>MLAVPNMRFGIFLLWWGWVLATESRMHWPGREVHEMSKKGRPQRQRREVHEDAHKQVSPILRRSPDITKSPLTKSEQLLRIDDHDFSMRPGFGGPAIPVGVDVQVESLDSISEVDMDFTMTLYLRHYWKDERLSFPSTNNLSMTFDGRLVKKIWVPDMFFVHSKRSFIHDTTTDNVMLRVQPDGKVLYSLRVTVTAMCNMDFSRFPLDTQTCSLEIESYAYTEDDLMLYWKKGNDSLKTDERISLSQFLIQEFHTTTKLAFYSSTGWYNRLYINFTLRRHIFFFLLQTYFPATLMVMLSWVSFWIDRRAVPARVPLGITTVLTMSTIITGVNASMPRVSYIKAVDIYLWVSFVFVFLSVLEYAAVNYLTTVQERKEQKLREKLPCTSGLPPPRTAMLDGNYSDGEVNDLDNYMPENGEKPDRMMVQLTLASERSSPQRKSQRSSYVSMRIDTHAIDKYSRIIFPAAYILFNLIYWSIFS[5x]

The family of ρ-type GABAA receptors includes potential therapeutic targets in several neurological conditions, and features distinctive pharmacology compared to other subtypes. Channels in this family share a common architecture, with each of the five subunits contributing to an extracellular domain (ECD) with 10 strands (β1–β10) and a transmembrane domain (TMD) with 4 helices (M1–M4). The orthosteric ligand-binding site is located at the subunit interface in the ECD, composed of loops A, B and C from the principal subunit and D, E and F from the complementary subunit. We implemented a modified human ρ1 GABAA receptor construct (ρ1-EM) with truncated loops in the N-terminus and intracellular domain and an inserted fluorescent protein to facilitate expression while largely preserving wild-type function.

The hydroxyl group at the C3 position of GABOB generates a stereogenic center, resulting in R and S enantiomeric forms; although (R)-GABOB is a modestly more potent anticonvulsant, the compound is applied clinically as a racemic mixture. Our cryo-EM dataset collected with GABOB contained particles in both partially-locked and desensitized states. In the presence of the agonist GABOB, one class (13% of resolved particles) corresponded to the desensitized state previously reported with GABA27. Consistent with our previous structure with GABA27, the desensitized state with GABOB exhibited further lockdown of loop C (4.3 Å S264-Cα translation) and rotation between the ECD and TMD (7.3°) relative to the partially-locked state. Interestingly, although all structures in this work contained ligands in the extracellular orthosteric site, local resolution in the ECD was relatively higher in the GABOB-desensitized state; in resting and partially-locked structures, resolution was similar between the domains, suggesting that channel activation is associated with both stabilization of the ECD and mobilization of the TMD. Densities for GABOB were clearly resolved in both the partially-locked and desensitized states. As in medical practice, we used a racemic mixture in our experiments, such that our cryo-EM densities likely contained both forms; indeed, either (R)- or (S)-GABOB could be modeled into the ligand density in either structure. The amino end was coordinated by an aromatic cage (Y219, Y262, Y268) as well as by E217 in the principal subunit, while the carboxylate end made electrostatic contacts with R125 and S189 in the complementary subunit. In all cases, T265 at the tip of loop C could make a hydrogen bond with the C3 hydroxyl, consistent with the demonstrated effect of this residue on potency of both GABOB forms.>ECSVDIQGNDQMQFNTNAITVDKSCKQFTVNLSHPGNLPKNVMGHNWVLSTAADMQGVVTDGMASGLDKDYLKPDDSRVIAHTKLIGSGEKDSVTFDVSKLKEG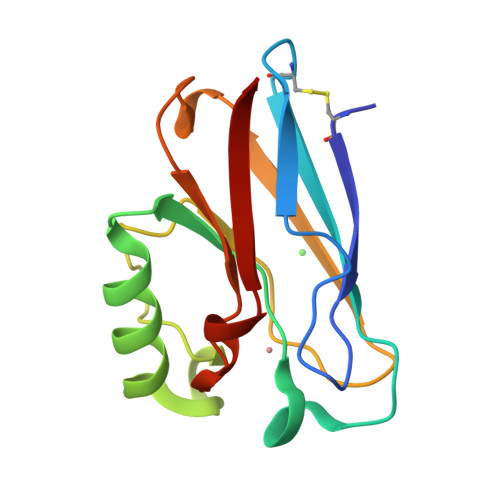EQYMFFCTFPGHSALMKGTLTLK[4x]(2~{S})-2-azanyl-4-[[(2~{S},3~{S},4~{R},5~{R})-5-[4-azanyl-5-(2-phenylethynyl)pyrrolo[2,3-d]pyrimidin-7-yl]-3,4-bis(oxidanyl)oxolan-2-yl]methylsulfanyl]butanoic acid | C23 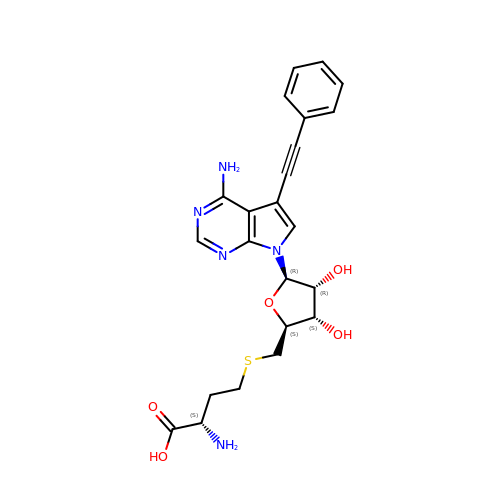H25 N5 O5 S | ARBIWWNISHROOL-XVZIYINBSA-N> SELLVNTKSGKVMGTRVPVLSSHISAFLGIPFAEPPVGNMRFRRPEPKKPWSGVWNASTYPNNCQQYVDEQFPGFSGSEMWNPNREMSEDCLYLNIWVPSPRPKSTTVMVWIYGGGFYSGSSTLDVYNGKYLAYTEEVVLVSLSYRVGAFGFLALHGSQEAPGNVGLLDQRMALQWVHDNIQFFGGDPKTVTIFGESAGGASVGMHILSPGSRDLFRRAILQSGSPNCPWASVSVAEGRRRAVELGRNLNCNLNSDEELIHCLREKKPQELIDVEWNVLPFDSIFRFSFVPVIDGEFFPTSLESMLNSGNFKKTQILLGVNKDEGSFFLLYGAPGFSKDSESKISREDFMSGVKLSVPHANDLGLDAVTLQYTDWMDDNNGIKNRDGLDDIVGDHNVICPLMHFVNKYTKFGNGTYLYFFNHRASNLVWPEWMGVIHGYEIEFVFGLPLVKELNYTAEEEALSRRIMHYWATFAKTGNPNEPHSQESKWPLFTTKEQKFIDLNTEPMKVHQRLRVQMCVFWNQFLPKLLNAT

Stabilization of Torpedo californica acetylcholinesterase by the divalent cations Ca+2, Mg+2, and Mn+2 was investigated. All three substantially protect the enzyme from thermal inactivation. Differential scanning calorimetry showed a single irreversible thermal transition. All three cations raise both the temperature of the transition and the activation energy, with the transition becoming more cooperative.

The crystal structures of the Ca+2 and Mg+2 complexes with Torpedo acetylcholinesterase were solved. A principal binding site was identified. In both cases, it consists of four aspartates (a 4D motif), within which the divalent ion is embedded, together with several water molecules. It makes direct contact with two of the aspartates, and indirect contact, via waters, with the other two. The ASSAM server retrieved 200 other proteins that display the 4D motif, in many of which it is occupied by a divalent cation. It is a very versatile motif, since, even though tightly conserved in terms of RMSD values, it can contain from one to as many as three divalent metal ions, together with a variable number of waters.> MDGEGFGELLQQAEQLAAETEGVTELPHVERNLQEIQQAGERLRSKTMTRTSQESANVKASVLLGSRGLDISHISQRLESLSAATTFEPLEPVKDTDIQGFLKNEKDNALLSAIEESRKRTFVMAEEYHRESMLVEWEQVKQRVLHTLLASGEDALDFTQESETSYISESGAPGRSSLDNVEMAYARQMYMYNEKVVSGHLQPSLVDLCTEAAERLDDKNVSDLWVMVKQMTDVPLIPASDTLKSRCSGQMQMAFVRQALNYLEQSYKNYTLISVFANLQQAQLGGVPGTYNLVRSFLNIRLPTPIPGLQDGEIEGYPVWALIYYCMRCGDLMAAQQVVNRAQHQLGDFKNCFQEYIHNKDRRLSPTTENKLRLHYRRAVRASTDPYKRAVYC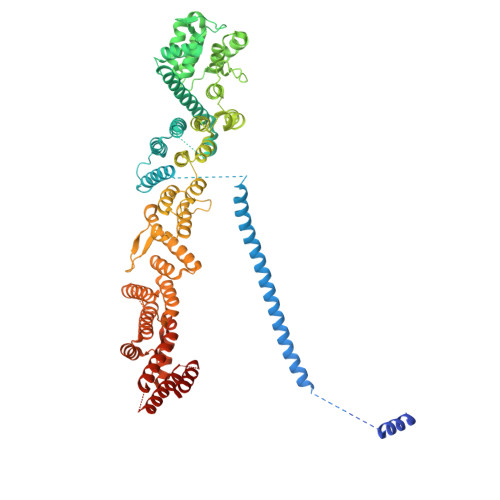IIGRCDVSDNHSEVADKTEDYLWLKLSQVCFEDEANSSPQDRLTLPQFQKQLFEDYGESHFAVNQQPYLYFQVLFLTAQFEAAIAFLFRLERTRCHAVHVALALFELKLLLKSTGQSAQLLSQEPGEPQGVRRLNFIRLLMLYTRKFEPTDPREALQYFYFLRNEKDNQGESMFLRCVSELVIESREFDMLLGKLEKDGSRKPGAIDKFTRDTKTIINKVASVAENKGLFEEAAKLYDLAKNPDKVLELTNKLLSPVVSQISAPQSNRERLKNMALAIAERYKSQGVSAEKSINSTFYLLLDLITFFDEYHAGHIDLSFDVIERLKLVPLSQDSVEERVAAFRNFSDEIRHNLSEILLATMNILFTQYKRLKGSGPTTLGRPQRVQEDKDSVLRSQARALITFAGMIPYRMSGDTNARLVQMEVLMN1~{H}-indol-6-yl-(4-methylpiperazin-1-yl)methanone | C14 H17 N3 O 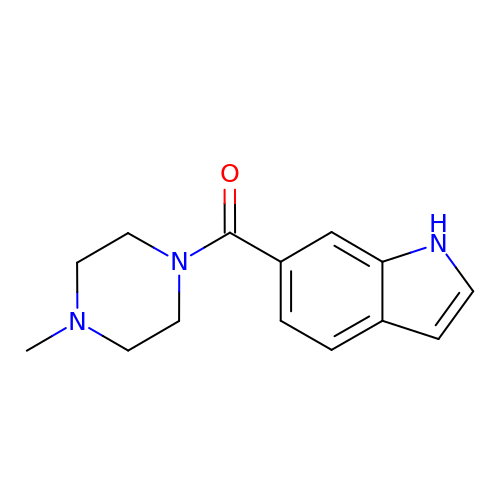| RQGONLHJHLGBII-UHFFFAOYSA-N> SNAMSVQLVKGVNLHVIPTEKYKTVRLLVRFNTRLNHETITKRTLLSSLMETNSLNYPNQVKLSERLAELYGASFGIGVSKKGNQHWFNISMNIVNDHYLQDSQVLAEAVDFLKEIIFAPNIQAGQFEAETFQREKENLKAYLESIVEDKQTYASLALQSVYFNQSEDQKIPSFGTVAALAEETAASLAAYYQKMLAEDQVDIFVLGDVNEAELVPLFKQLPFTPREEGKAAIFYNQPIRNVIEERTEREVLAQSKLNLAYNTDIYYG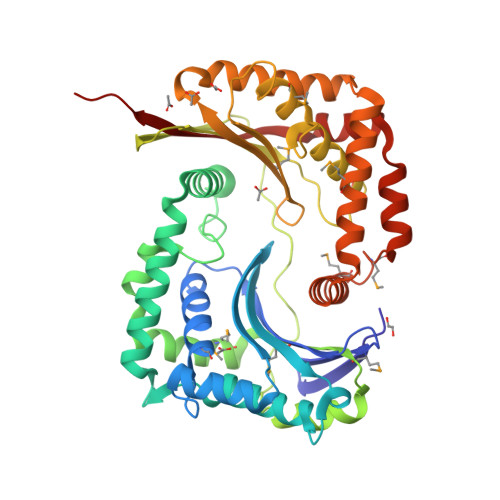DSYYFALQVFNGIFGGFPHSKLFMNVREKEHLAYYASSSIDTFRGFMTVQTGIDGKNRNQVLRLISTELENIRLGKIRELEIEQTKAMLKNQYILALDNAGAWLEKEYLNELMPQTMLTAEEWIARINAVTIPEIQEVAKRLELQAIFFLEGETEND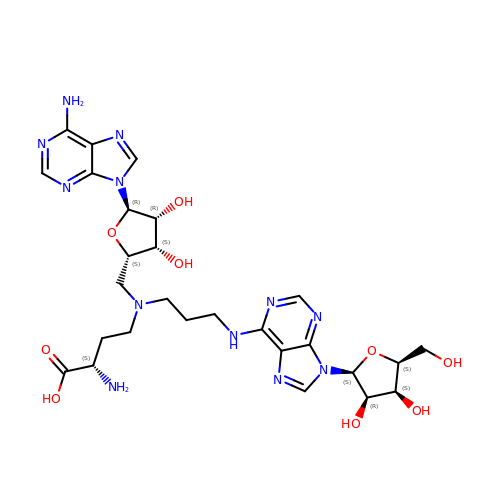(2~{S})-4-[[(2~{S},3~{S},4~{R},5~{R})-5-(6-aminopurin-9-yl)-3,4-bis(oxidanyl)oxolan-2-yl]methyl-[3-[[9-[(2~{S},3~{R},4~{S},5~{S})-5-(hydroxymethyl)-3,4-bis(oxidanyl)oxolan-2-yl]purin-6-yl]amino]propyl]amino]-2-azanyl-butanoic acid | C27 H38 N12 O9 | BNMNWGQODJWABC-JIDNCIPASA-N> I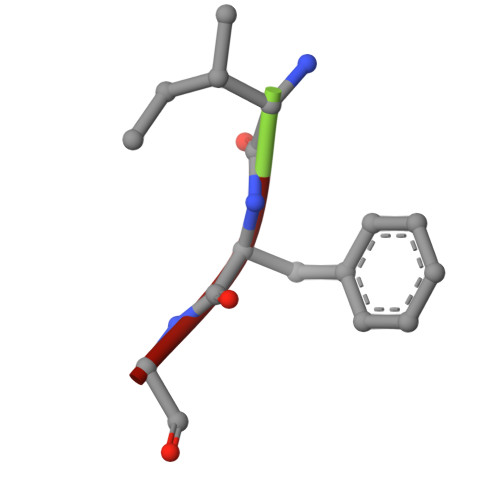FG PIN2/TRF1-interacting telomerase inhibitor 1 (PinX1) functions as a telomerase inhibitor and tumor suppressor. We determined the crystal structure of the TRFH (TRF homology) domain of TRF1 in complex with a short TRF1-binding motif of PinX1 and revealed that PinX1 bound to TRF1 via the F-X-L-X-P motif, providing a structural basis of how PinX1 is recruited to the telomeric region by TRF1. We demonstrated that PinX1 is directly associated with and inhibits telomerase activity by TID (telomerase inhibitory domain) with crucial lysine residues clustered in PinX1292-301.

We have reported the crystal structure of the telomeric TIN2-TRF1 complex previously, revealing that the short TBM (TRFH-binding motif) of TIN2 directly binds to the TRFH of TRF1.2 Notably, an 11-residue fragment of PinX1 (R287-D-F-T-L-K-P-K-K-R-R297), referred to as PinX1TBM, closely resembles TIN2TBM, indicating that it may bind to TRF1TRFH in the same fashion as TIN2TBM does. To provide direct and independent evidence of the PinX1-TRF1 interaction, we purified a high-quality TRF1TRFH-PinX1TBM complex and determined its crystal structure at a resolution of 2.7 Å. The structure showed that TRF1TRFH formed homodimers, with each TRF1TRFH interacting with one PinX1TBM peptide. The electron density map demonstrates that the PinX1TBM peptide assumes a well-defined conformation. Similar to the TIN2TBM-TRF1TRFH interface, hydrophobic contacts are essential for the interaction between PinX1TBM and TRF1TRFH. L291 of PinX1 was deeply buried in a pocket formed by L86, R102, C126, and T130 of TRF1, supporting previous findings that the L291E mutation in PinX1 disrupts its ability to be bound and recruited by TRF1.2,3 The aromatic side-chain of F289 of PinX1 packed against a hydrophobic surface of TRF1 and the proline ring of PinX1 P293 stacked with TRF1 F142. Notably, except for R297 of PinX1 that is engaged in electrostatic interactions with E146 and E192 of TRF1, all other basic residues in PinX1TBM (K292, K294, K295, R296, and K299) extended outward from the interface and did not contribute to the interaction with TRF1. PinX1MUT (A292-P-L-G-R-R-G-V-Q-S301) almost completely abolished PinX1 RTI in the TRAP assay, although the TRFH binding capability was unaffected, suggesting that lysine residues in PinX1292-301 are essential for the telomerase inhibitory activity of PinX1. As a natural suppressor of telomerase, PinX1 represents a potential strategy for curtailing cancer progression by targeting telomerase. This study reported the crystal structure of the TRF1TRFH-PinX1TBM complex and confirmed that PinX1 was recruited to the telomere by TRF1 predominantly via the binding to the F-X-L-X-P motif, highlighting its tumor-suppressive impact on CESC.

>[4x]EEEEEDAGLVAEAEAVAAGWMLDFLCLSLCRAFRDGRSEDFRRTRNSAEAIIHGLSSLTACQLRTIYICQFLTRIAAGKTLDAQFENDERITPLESALMIWGSIEKEHDKLHEEIQNLIKIQAIAVCMENGNFKEAEEVFERIFGDPNSHMPFKSKLLMIISQKDTFHSFFQHFSYNHMMEKIKSYVNYVLSEKSSTFLMKAAAKVVESKRT;>SGRDFTLKPKKRRGKKKLQK[4x]>MPVLENRAAQGDITAPGGARRLTGDQTAALRDSLSDKPAKNIILLIGDGMGDSEITAARNYAEGAGGFFKGIDALPLTGQYTHYALNKKTGKPDYVTDSAASATAWSTGVKTYNGALGVDIHEKDHPTILEMAKAAGLATGNVSTAELQDATPAALVAHVTSRKCYGPSATSEKCPGNALEKGGKGSITEQLLNARADVTLGGGAKTFAETATAGEWQGKTLREQAQARGYQLVSDAASLNSVTEANQQKPLLGLFADGNMPVRWLGPKATYHGNIDKPAVTCTPNPQRNDSVPTLAQMTDKAIELLSKNEKGFFLQVEGASIDHQDHAANPCGQIGETVDLDEAVQRALEFAKKEGNTLVIVTADHAHASQIVAPDTKAP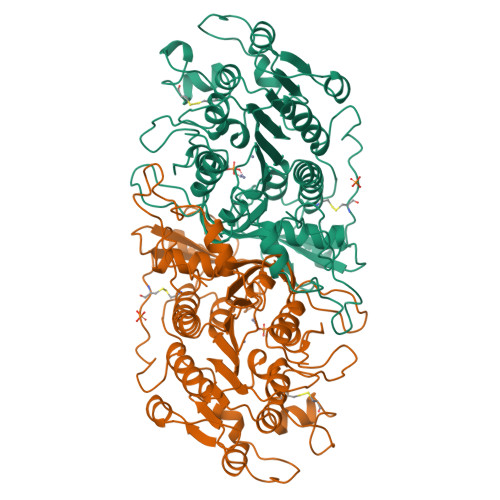GLTQALNTKDGAVMVMSYGNSEEDSQEHTGSQLRIAAYGPHAANVVGLTDQTDLFYTMKAALGLK[2x]> NECLGTIGPVTPLDASDFALDIRMPGVTPKESDTYFCMSMRLPVDEEAFVIDFKPRASMDTVHHMLLFGCNMPSSTGSYWFCDEGTCTDKANILYAWARNAPPTRLPKGVGFRVGGETGSKYFVLQVAYGDISAFRDNHKDCSGVSVHLTRVPQPLIAGMYLMMSVDTVIPPGEKVVNADISCQYKMYPMHVFAYRVHTHHLGKVVSGYRVRNGQWTLIGRQNPQLPQAFYPVEHPVDVTFGDILAARCVFTGEGRTEATHIGGTSSDEMCNLYIMYYMEAKYALSFMTCTKNVAPDMFRTIPAEANIPIPV

Two enzymes, peptidylglycine α-hydroxylating monooxygenase (PHM; EC 1.14.17.3) and peptidyl-α-hydroxyglycine α-amidating lyase (PAL; EC 4.3.2.5) working sequentially are the only proteins known to catalyze this reaction. PHM, a two Cu enzyme, catalyzes the stereospecific hydroxylation of the glycine Cα of peptidylglycine substrates. The two copper atoms in PHM, CuH, and CuM (located in the N- and C-subdomains, respectively), each use a single reducing equivalent from ascorbate to catalyze the reduction of molecular oxygen for the hydroxylation of the Cα of glycine at the carboxy-terminus of the peptide substrate. Crystallographic data on apo wild-type PHM and on several crystal forms of three CuH mutants (H107A, H108A, and H172A) presented here show that the copper ions are required not only for the catalytic steps but also for substrate binding and for locking the overall conformation of PHM in a configuration that is catalytically active.

Even though the molecule does not contain copper in the CuH site, copper at the CuM site has the same coordination and geometry as the wild-type. The CuH site displays only the minimum changes compatible with the mutation and the absence of its copper (RMSD 0.61 Å). The N- and C-subdomains come closer by a small displacement (<0.5 Å). More surprising, although it has no copper in the CuH site, the conformation of the two remaining histidines in this site, His 107 and His 108, is almost unmodified from that of wild-type PHM and the CuM site retains the same coordination of the copper observed in wild-type PHM.>[2x]PPYTVVYFPVRGRCAALRMLLADQGQSWKEEVVTVETWQEGSL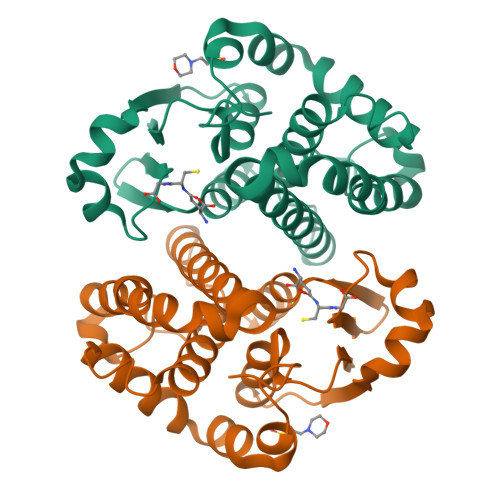KASCLYGQLPKFQDGDLTLYQSNTILRHLGRTLGLYGKDQQEAALVDMVNDGVEDLRCKYISLIYTNYEAGKDDYVKALPGQLKPFETLLSQNQGGKTFIVGDQISFANYNLLDLLLIHEVLAPGCLDAFPLLSAYVGRLSARPKLKAFLASPEYVNLPINGNGKQ>SQKNFLCDTGAYELVGAFLENYLREFENDEFRHNLYKYYSENSIFTLTCNYNVVQNHQTPKILQRLSKYNRHARNLRNKDYSKASDGVFFGCTYIVEILLQLPRVTHDFHSLQTDVMHYNGKGAVIYVAGLLRDEPPSTRNGHGSKTDIGGVLLGFSRQFVVTFDEANLGLGKRARRLKIANERLHITNPSKTAIRNAFSVNFPDP[2x];>MDSDLKAKVESCARTADTFTRLYYASVDNRRQQIGRLYLDNATLSWNGNGAIGRQ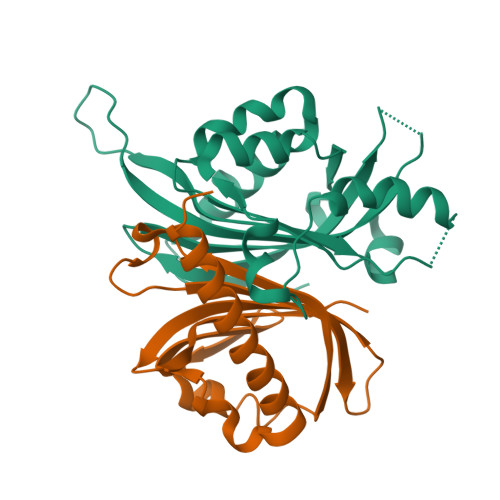MIESYFQELPSSNHQLNTLDAQPIVDQAVSNQLAYLIMASGSVKFADQQLRKFQQTFIVTAENDKWKVVSDCYRMQEV[2x]3-methyl-N-[(pentyloxy)carbonyl]-L-valyl-(4R)-4-[(3-chloro-7-methoxyquinoxalin-2-yl)oxy]-N-[(1R,2S)-2-ethenyl-1-{[(1-methylcyclopropyl)sulfonyl]carbamoyl}cyclopropyl]-L-prolinamide | C36 H49 Cl N6 O9 S | 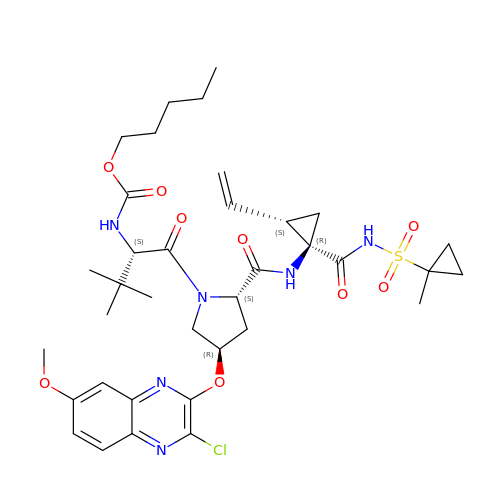GCSLYGDUYMRXAE-BTMIYQIWSA-N ethyl 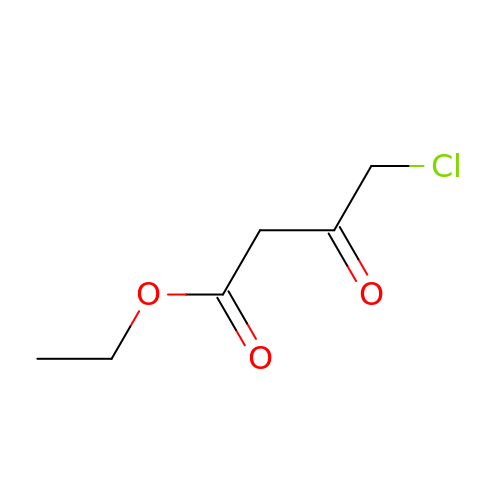4-chloranyl-3-oxidanylidene-butanoate | C6 H9 Cl O3 | OHLRLMWUFVDREV-UHFFFAOYSA-N5'-O-(N-(L-seryl)-sulfamoyl)N3-methyluridine 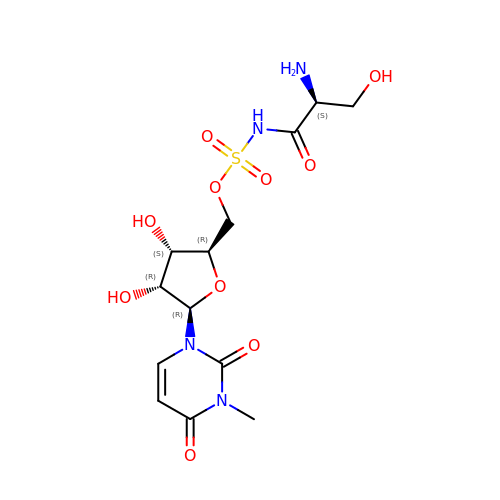| C13 H20 N4 O10 S | FDYLXUQGMZNPQQ-IXKMEIRJSA-N GapR is an essential NAP in Caulobacter crescentus involved in DNA replication, chromosome segregation and cell division. In this paper we present three crystal structures of GapR from C. crescentus, crystallised in the presence of double-stranded DNA with a sequence from the origin of chromosome replication. In all three structures, GapR adopts the same overall tetramer ring form as seen by Guo et al., albeit with small but important increases in the diameter of the central channel. DNA could not be visualized in any of our three structures, but DNA could be detected in gel electrophoresis, indicating that DNA is present in the crystals.

The same crystallization condition also produced crystals with a second morphology, which were of the space group P2221. The diffraction from these crystals displayed severe anisotropy and had resolution limits between 2.0 and 2.7 Å. In this crystal, GapR is a dimer in the asymmetric unit, with the tetramer again being formed by crystallographic symmetry. The tetramer could be overlaid onto the I4132 tetramer with a root-mean-square deviation (rmsd) of 1.5 Å. The main difference between GapR in the three crystal forms arises from slight changes in the orientation of helix three, which results in minor variations in the size of the central channel.

>[2x]MHHHHHHHHPDLGTGSENLYFQGAMADDAIPHTDVLNSTAQGQLKSIIERVERLEVEKAEIMEQIKEVYAEAKGNGFDVKVLKKVVRIRKQDRAKRQEEDAILDLYLSAIGEI> GTDLITLEMVFAANLNQDKSSCEAILPFLNEYAKTYGMKEERAMAHF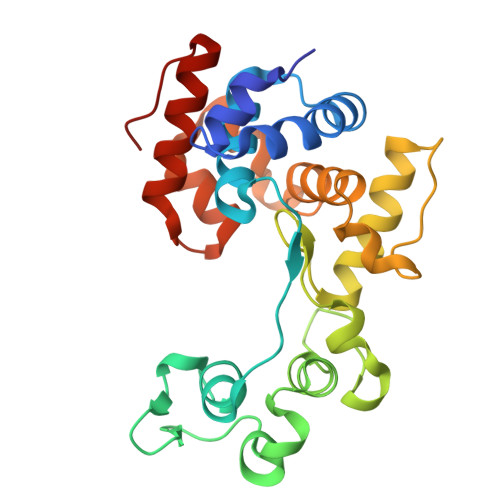LSQVGHESNFKPVSENLRYSPKGMRKIFGCKGGSKNYDPILDDAKEGRLRPKLWTHESDYAFNPVALGNYVYANRPGSKNGDESSGDGYKYRGRGLIQITHKDAYIKFTEAHNAANPSDQKDFLASPDDILTLRYATSSAYFFWFIYKKSFNLHSTACTGTVKEVTKIVNGGYAGYADRLKRFNAVAAVIGIDGARE Protease VhaC is a multi-domain enzyme composed of a CM containing an activator domain and a peptidase domain, a PKD-like domain and a PPC domain. Sequence analysis using Conserved Domain Search showed that VhaC is a multi-domain protein containing an activator domain (Ser70-Tyr346), a peptidase domain (Gly347-Val605), a PKD-like domain (Ser606-Ala698), and a PPC domain (Leu699-Gln814). VhaC had activity toward various types of collagens, showing that it is a collagenase. Structural and biochemical analyses and molecular dynamics studies reveal that triple-helical collagen is initially recognized by the activator domain, followed by subsequent cleavage by the peptidase domain along with the closing movement of CM.

However, only the crystal structure of CM was solved to 1.8 Å resolution. The CM crystal belongs to the P 21 space group with one molecule per asymmetric unit. The CM structure contains residues from Cys78 to His609, suggesting that the N-terminal signal peptide and propeptide in the CM precursor are cleaved off during enzyme maturation. In this study, the crystal structure of the CM was solved, it having a more contracted saddle-shaped architecture and lacking the catalytic helper subdomain, when compared to that of Clostridium collagenase ColG, the only CM structure in the M9 family. Unexpectedly, the structure data show that the CM molecule binds two peptides (peptide P1: 24-EPSQQVTEIYQHHA-37; peptide P2: 48-DYAPTKLLPQQP-59) derived from the propeptide of VhaC via hydrogen bonds and hydrophobic interactions. While peptide P2 entirely binds to the activator domain, the N-terminus of peptide P1 binds to the activator domain and its C-terminus extends and binds to the catalytic center of the peptidase domain. Correspondingly, in the CM structure of VhaC, the C-terminal residues of peptide P1 also bind to the conserved Gly441-Gly442 motif, representing the S1′ peptide recognition site. Therefore, peptides P1 and P2 can be regarded as substrate analogues in the CM structure, which may provide clues for the recognition pattern of collagen substrates in CM. In the CM structure, a catalytic Zn2+ is tetrahedrally coordinated by the side chains of His477, His481, and Glu505 from the peptidase domain, as well as the side chain of a histidine from peptide P1 instead of the characteristic water molecule observed in 2Y5022. In addition, a Ca2+ ion, located on the left rim of the active-site cleft and 14.2 Å away from the catalytic Zn2+ ion, is coordinated by the backbone oxygens of Gly485, Leu489, and Gly491 and the side chain of Glu446.

> MELKNLTVAIATFFASTNALALSEPSQQVTEIYQHHAHQNGNDRALPDYAPTKLLPQQPKPTLRTLSTRSAEQAANVCDVEAFTSNSSNDVLNAIKTQGASCVNALFSAESRIQEAAFESGHMYNIAKHTTDLAKAYAGGGSDELEALFLYLRAGYYAEFYNSKVSFLSWVTPAVKEAVDAFVNNANFYENSDPHGKVLSEVIITMDSAGLQHAYLPQVTQWLTRWDSQYAQNWYMRNAVNGVFTILFGGQWNEQFVQTIGNQTELAKALGDFALRSSAIGASDEFMAANAGRELGRLTKYSGSASSTVKSKLTEIFAQYEMYGRGDAIWLGAADTVSYYADCSDYGICNFESQLKGLVLSQSYTCSPTIRILSQNMTQDQHVAACSKMGYEEGYFHTSLETGRQPVADDYNTQLQVNIFDSSDDYGKYAGPIFNISTNNGGMYLEGDPATPGNIPNFVAYEAPYANPDHFVWNLEHEYVHYLDGRFDLYGGFGHPTERIVWWSEGIAEYVSKENDNQAAIDTIKDGSTFTLSEIFETSYDGFDVDRIYRWGYLAVRFMFERHKDDVNQMLIETRQGNWANYKATINQWAILYQSEFEQWQQALVLEHHHHHH;> EPSQQVTEIYQHHA;> DYAPTKLLPQQP> GSHEMIKSLQHRPSPSAEEWELIHVVTEAHRSTNAQGSHWKQKRKFLPEDIGQSPMASMPDGDKVDLEAFSEFTKIITPAITRVVDFAKKLPMFSELPCEDQIILLKGCCMEIMSLRAAVRYDPESETLTLSGEMAVKREQLKNGGLGVVSDAIFDLGKSLSAFNLDDTEVALLQAVLLMSSDRTGLICVDKIEKCQETYLLAFEHYINYRKHNIPHFWPKLLMKVTDLRMIGACHASRFLHMKVECPTELFPPLFLEVFEDQEV;> MKKGSANE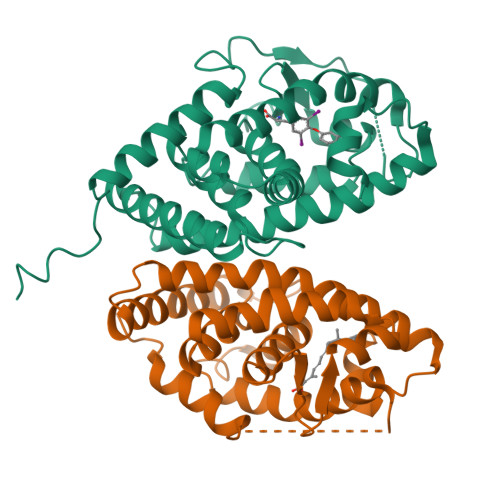DMPVERILEAELAVEPKTETYVEANMGLNPSSPNDPVTNICQAADKQLFTLVEWAKRIPHFSELPLDDQVILLRAGWNELLIASFSHRSIAVKDGILLATGLHVHRNSAHSAGVGAIFDRVLTELVSKMRDMQMDKTELGCLRAIVLFNPDSKGLSNPAEVEALREKVYASLEAYCKHKYPEQPGRFAKLLLRLPALRSIGLKCLEHLFFFKLIGDTPIDTFLMEMLEAPHQMTMT> GSHMVPISFVFNRFPRMVRDLAKKMNKEVNFIMRGEDTELDRTFVEEIGEPLLHLLRNAIDHGIEPKEERIAKGKPPIGTLILSARHEGNNVVIEVEDDGRGIDKEKIIRKAIEKGLIDESKAATLSDQEILNFLFVPGFSTKEKVSEVSGRGVGMDVVKNVVESLNGSISIESEKDKGTKVTIRLPLTLAIIQALLVKVNNLVYAIPIANIDTILSISKEDIQRVQDRDVIVIRGEVIPVYRLWEVLQIEHKEELEEMEAVIVRVGNRKYGIVVDDLLGQDDIVIKSLGKV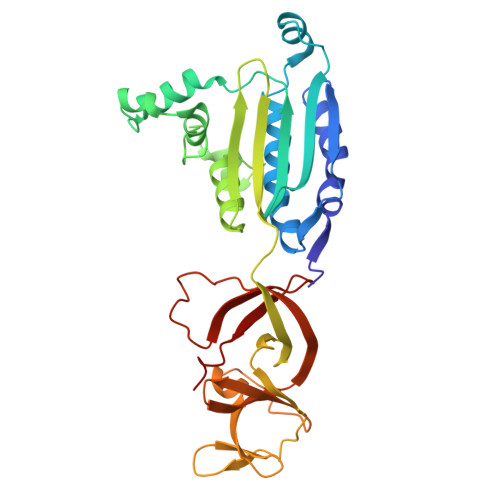FSEVKEFSGAAILGDGSIALIINVSGIV> AGGGTTAGGGTT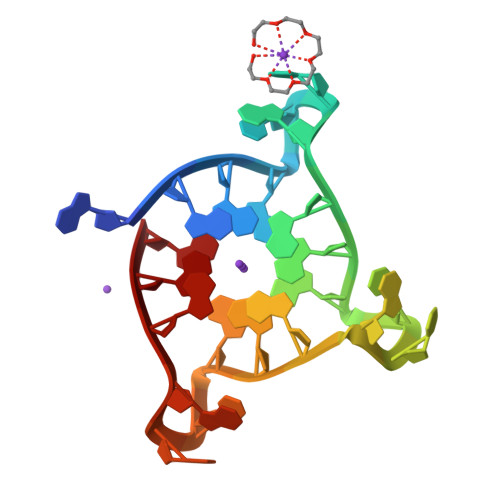AGGGTTAGGG2-[3-METHYL-4-(N-METHYL-GUANIDINO)-BUTYRYLAMINO]-3-(4-PHENYLETHYNYL-PHENYL)-PROPIONIC 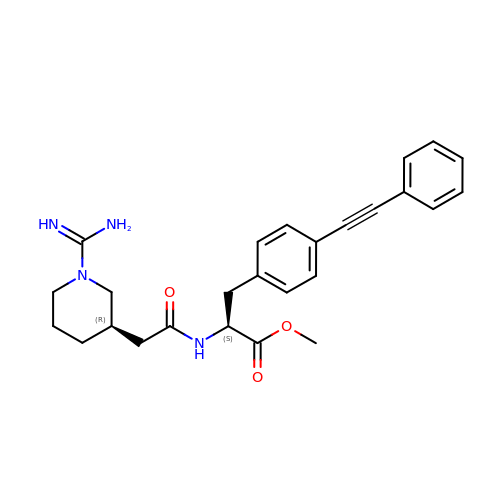ACID METHYL ESTER | C26 H30 N4 O3 | MRNGXYMKYHNMLV-PKTZIBPZSA-N>[3x]MKIDPIRETTDEARALARQLLEAARHASLGTLDPETGVPLVTRIALQTDADGVPLALLAGLAAHARALAVDPRAGLLIAAEAAKGDAMTHARLSILGRAVPAEPDE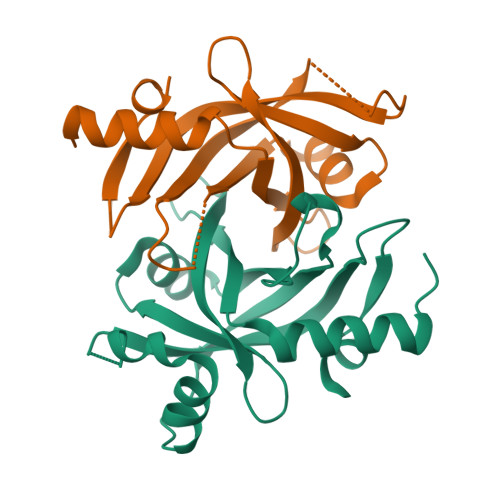NRRARWLERDPKAKVYLDLPDFRFWRIEPVSGLLNAGFGQAFKLTASDMLKPPAE>GHHHHHHGENLYFQGASLTEIEHLVQSVCKSYRETCQLRLEDLLRQRSNIFSREEVTGYQRKSMWEMWERCAHHLTEAIQYVVEFAKRLSGFMELCQN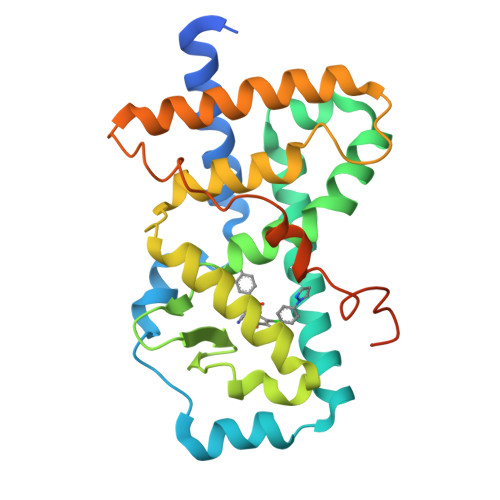DQIVLLKAGAMEVVLVRMCRAYNADNRTVFFEGKYGGMELFRALGCSELISSIFDFSHSLSALHFSEDEIALYTALVLINAHRPGLQEKRKVEQLQYNLELAFHHHLCKTHRQSILAKLPPKGKLRSLCSQHVERLQIFQHLHPIVVQAAFPPLYKELFS[2x]> SDKIIHLTDDSFDTDVLKADGAILVDFWAEWCGPCKMIAPIL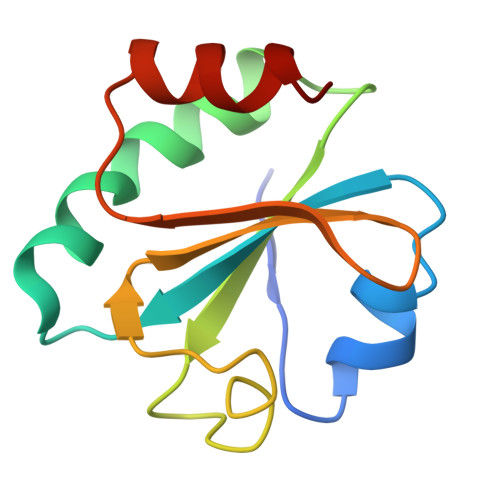DEIADEYQGKLTVAKLNIDQNPGTAPKYGIRGIPTLLLFKNGEVAATKVGALSKGQLKEFLDANLA> MGHHHHHHSGENLYFQGASMRTLLIRYILWRNDN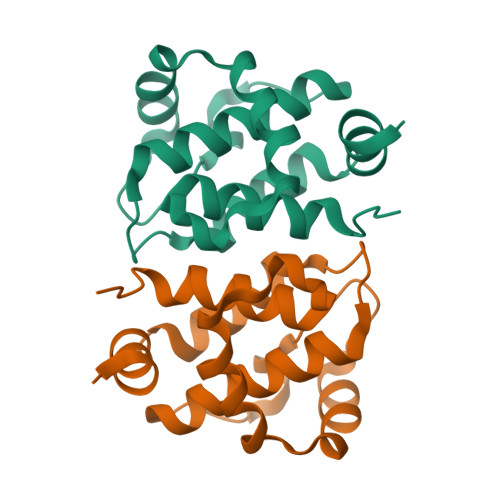DQTYYNDDFKKLMLLDELVDDGDVCTLIKNMRMTLSDGPLLDRLNQPVNNIEDAKRMIAISAKVARDIGERSEIRWEESFTILFRMIETYFDDLMIDLYGEK>SVSEIQLMH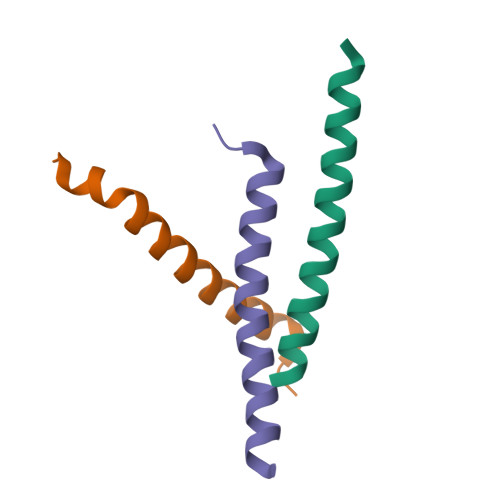NLGKHLNSMERVEWLRKKLQDVHNF[3x]>[2x]GSHMAWPGPLLLKDRKGRAYLVFPKEGGVFHHHKGSVPHEALLEAGPGGVVRTHLGEELSVHRPTLEEYLLHMKRSATPTYPKDASAMVTLLDLAPGMRVLEAGTGSGGLTLFLARAVGEKGLVESYEARPHHLAQAERNVRAFWQVENVRFHLGKLEEAELEEAAYDGVALDLMEPWKVLEKAALALKPDRFLVAYLPNITQVL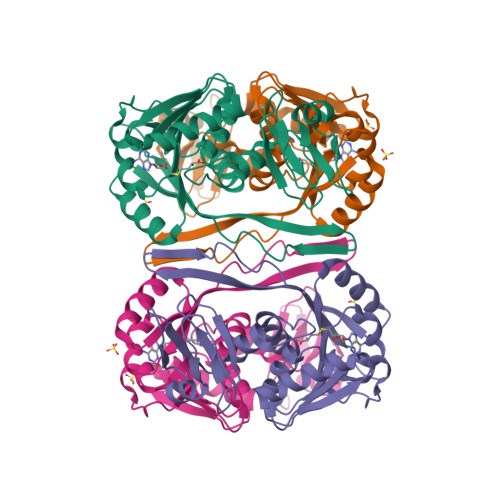ELVRAAEAHPFRLERVLEVGWREWEVRLPVAHPRFQQVGHTAFLVALRRWKGS>[3x]SDGPGSAEIVTEEQGTVVQQQPAPAPTALATLATASTGKSVEQEWMTFFSYHTSINWSTVESQGKILYSQALNPSINPYLDHIAKLYSTWSGGIDVRFTVSGSGVFGGKLAALLVPPGVEPIESVSMLQYPHVLFDARQTEPVIFTIPDIRKTLFHSMDETDTTKLVIMVYNELINPYENGVENKTTCSITVETRPSADFTFALLKPPGSLIKHGSIPSDLIPRNSAHWMGNRWWSTISGFSVQPRVFQSNRHFDFDSTTTGWSTPYYVPIEIKIQGKVGSNNKWFHVIDTDKALVPGIPDGWPDTTIPDETKATNGNFSYGESYRAGSTTIKPNENSTHFKG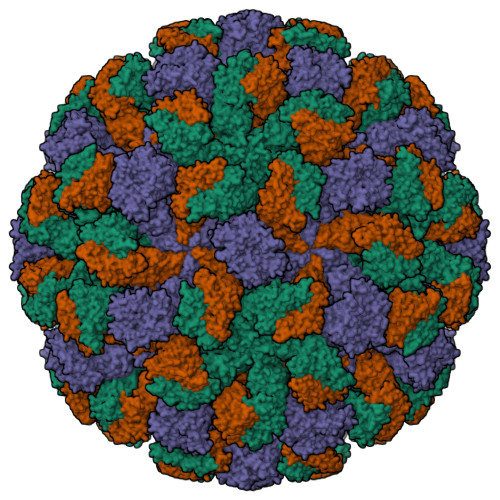TYICGTLSTVEIPENDEQQIKTEAEKKSQTMYVVTADFKDTIVKPQHKISPQKLVVYFDGPEKDLTMSATLSPLGYTLVDEQPVGSVSSRVVRIATLPEAFTQGGNYPIFYVNKIKVGYFDRATTNCYNSQILMTSQRLAEGNYNLPPDSLAVYRITDSSSQWFDIGINHDGFSYVGLSDLPNDLSFPLTSTFMGVQLARVKLASKVKAHTITAK>[12x]MNTLDTLPVHPRTGLRAIGMGKRGPIWPVMGASDDHKDDAPTLTYSQARNRADEVHARMEQIAELDKPTDEENEEFRALGAEFDSLVNHMSRLERAAELARVRSTHEQIGKPQSGGQRRMRVEAGSSQGGRGDYDRDAILEPDSIEDCRFRDPWNLSEMRTFGRDAEEVKGELRARALSAIEKMQGASDNVRAAATHIIERFDDEDST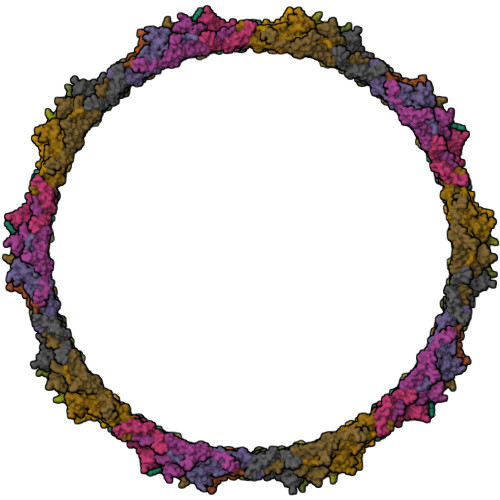LARQCLATSSPAYLRAWSKMARNPHAAILTEEEKRAINEVRAMGLTKADGGYLVPFQLDPTVIITSNGSLNDIRRFARQVVATGDVWHGVSSAAVQWSWDAEFEEVSDDSPEFGQPEIPVKKAQGFVPISIEALQDEANVTETVALLFAEGKDELEAVTLTTGTGQGNQPTGIVTALAGTAAEIAPVTAETFALADVYAVYEQLAARHRRQGAWLANNLIYNKIRQFDTQGGAGLWTTIGNGEPSQLLGRPVGEAEAMDANWNTSASADNFVLLYGNFQNYVIADRIGMTVEFIPHLFGTNRRPNGSRGWFAYYRMGADVVNPNAFRLLNVETAS>FNLPPGNYKKPKLLYCSNGGHFLRILPDGTVDGTRDRSDQHIQLQLSAESVGEVYIKSTETGQ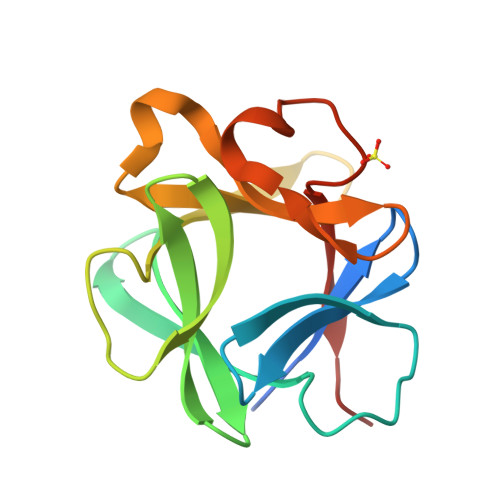YLAMDTDGLLYGSQTPNEECLFLERLEENHYNTYISKKHAEKNWFVGLKKNGSCKRGPRTHYGQKAILFLPLPVSSD[4x]>[3x]MNHKVHHHHHHIEGRHMPLNNYLHVFYYSWYGNPQFDGKYIHWNHPVLEHWDPRIAKNYPQGRHNPPDDIGSSFYPELGSYSSRDPSVIETHMRQMRSASIGVLALSWYPPDVNDENGEPTDNLVPTILDKAHKYNLKVTFHIEPYSNRDDQNMYKNVKYIIDKYGNHPAFYRYKTKTGNALPMFYVY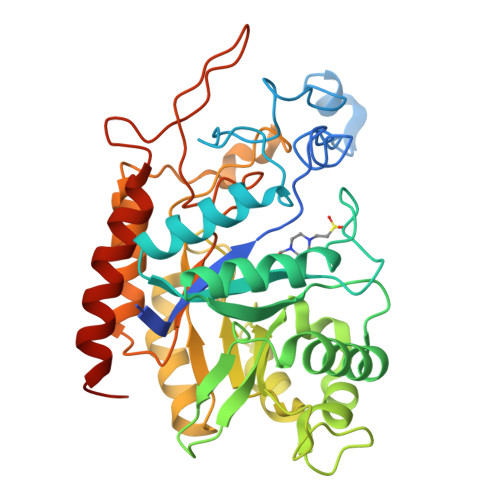DSYITKPEKWANLLTTSGSRSIRNSPYDGLFIALLVEEKHKYDILQSGFDGIYTYFATNGFTYGSSHQNWASLKLFCDKYNLIFIPSVGPGYIDTSIRPWNTQNTRNRINGKYYEIGLSAALQTRPSLISITSFNEWHEGTQIEKAVPKRTSNTVYLDYRPHKPGLYLELTRKWSEKYSKERATYALDRQLPVS~{N}-[6-methyl-2-[(2~{S})-2-[3-(3-methylpyrazin-2-yl)-1,2-oxazol-5-yl]pyrrolidin-1-yl]pyrimidin-4-yl]-1,3-thiazol-2-amine 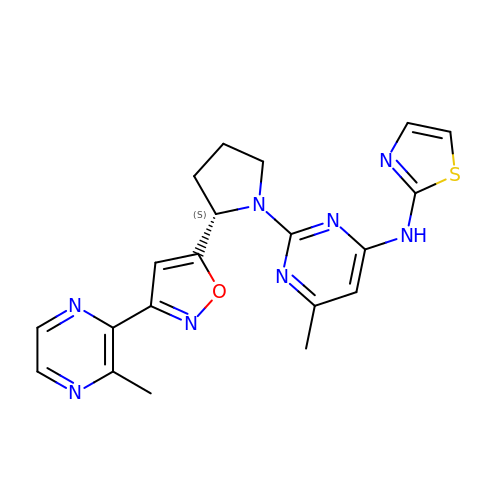| C20 H20 N8 O S | FBNXQICSZNRHCD-HNNXBMFYSA-N> ASMWERVKSIIKSSLAAASNI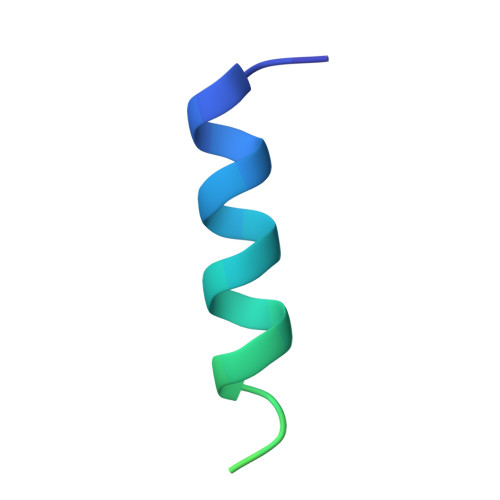PGPIGVAASGISGLSALFEGFGF>MRHLKSGRKLNRHSSHRLALYRNQAKSLLTHGRITTTVPKAKELRGFVDHLIHLAKRGDLHARRLVLRDLQDVKLVRKLFDEIAPRYRDRQGGYTRVLKLAERR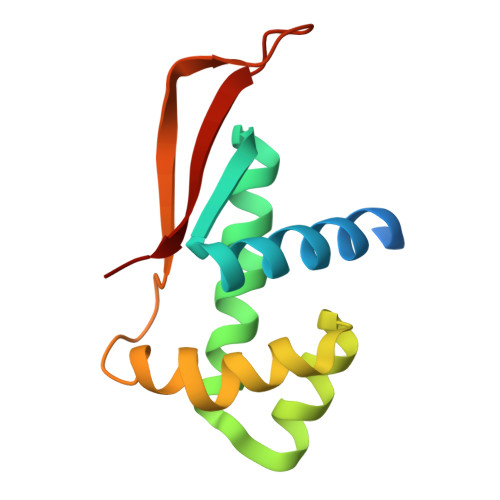RGDGAPLALVELVE[9x]>MEHICGTSRIAGFRFSLYPMTDDFISVIKSALAATDTSKVWTKTDHISTVLRGSIDHVFDAAKAIYLHAANSEQHIVMNGTFSIGCPGDTQGDTYLSKGDKRVNEDAVRGLKAEAPCQFALYPMNEPDYMGLIMEAVDIAKAQ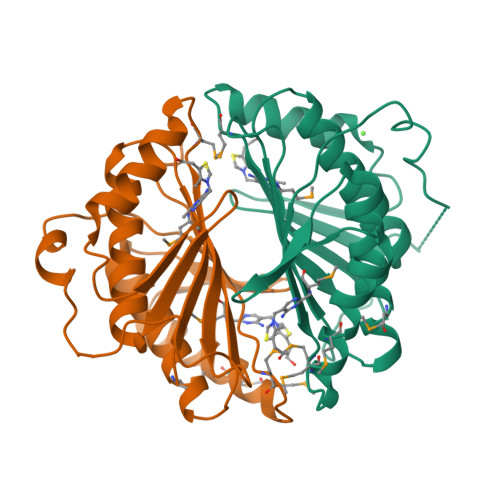GTFVQGVHYASELDGDAHDVFSTLEAVFRMAEQQTNHITMTVNLSANSPSRKNRKQG[2x]1-[(1R)-1-cyclohexyl-2-(methylamino)-2-oxoethyl]-L-proline | C14 H24 N2 O3 | 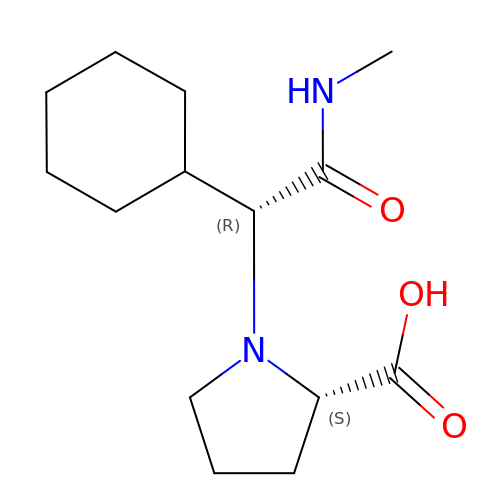OCMCWMIWKWLBKH-NWDGAFQWSA-N> GMSPNYDKWEMERTDITMKHKLGGGQYGEVYEGVWKKYSLTVAVKTLKEDTMEVEEFLKEAAVMKEIKHPNLVQLLGVCTREPPFYIITEFMTYGNLLDYLRECNRQEVNAVVLLYMATQISSAMEYLEKKNFIHRDLAARNCLVGENHLVKVADFGLSR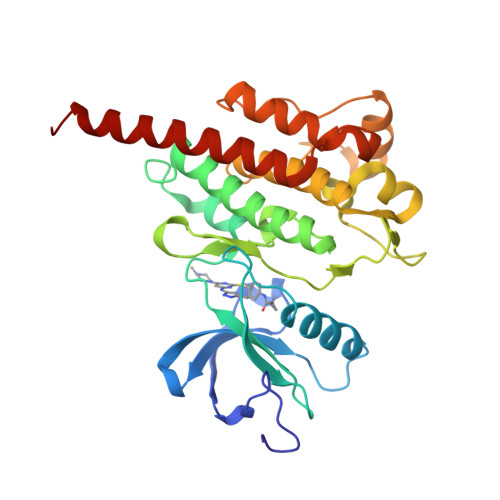LMTGDTYTAPAGAKFPIKWTAPESLAYNKFSIKSDVWAFGVLLWEIATYGMSPYPGIDLSQVYELLEKDYRMERPEGCPEKVYELMRACWQWNPSDRPSFAEIHQAFETMFQESSISDEVEKELGKQ>PFTYSIEATRNLATTERCIQDIRNAPVRNRSTQFQLAQQNMLAYTFGEVIPGFASAGINGMDYRDVIGRPVENAVTEGTHFFRDDFRVDSNAKAKVAGDIFEIVSSAVMWNCAARWNSLMVGEGWRSQPRYSRPTLSPSPRRQVAVLNLPRSFDWVSLLVPESQEVIEEFRAGLRKDGLGLPTSTPDLAVVVLPEEFQNDEMWREEIAGLTRPNQILLSGAYQRLQGRVQPGEISLAVAFKRSLRSDRLYQPLYEANVMQLLLEGKLGAPKVEFEVHTLAPEGTNAFVTYEAASLYGLAEGRSAVHRAIRELYVPPTAADLAR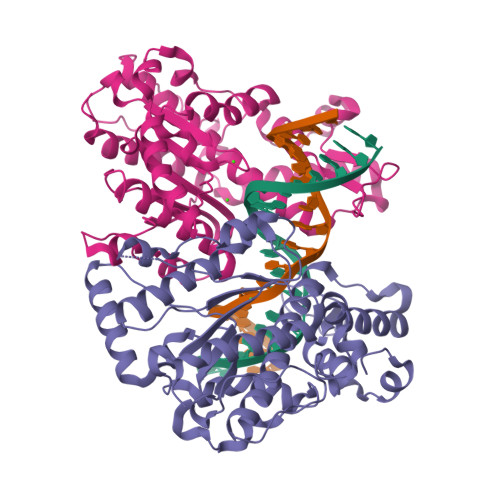RFFAFLNERMELVNG[4x]>[2x]MSLSRGCRGAKTQVISPSKRARPAEESRKRLRFARLSEHATAPTKGSERAAGYDLYSAYDYTVLPMEKAIVKTDIQIALPSGCYGRVAPRSGLAAKHFIDVGAGVIDEDYRGNVGV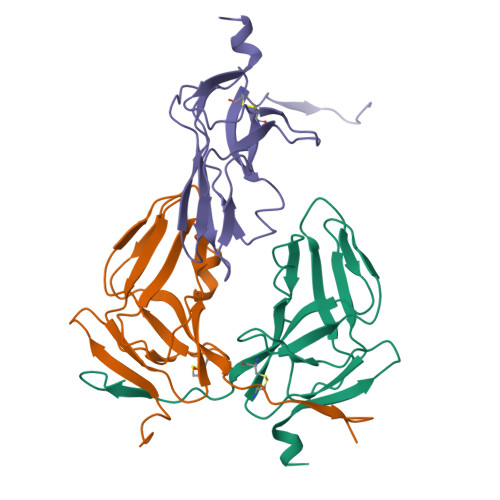VLFNFGKEKFEVKKGDRIAQLICERIFYPEIEEVQVLDDTKRGSGGFGSTGTN N~1~-butyl-5-cyano-N~3~-{(1S,2R)-1-(3,5-difluorobenzyl)-2-hydroxy-3-[(3-methoxybenzyl)amino]propyl}-N~1~-methyl-1H-indole-1,3-dicarboxamide | C34 H37 F2 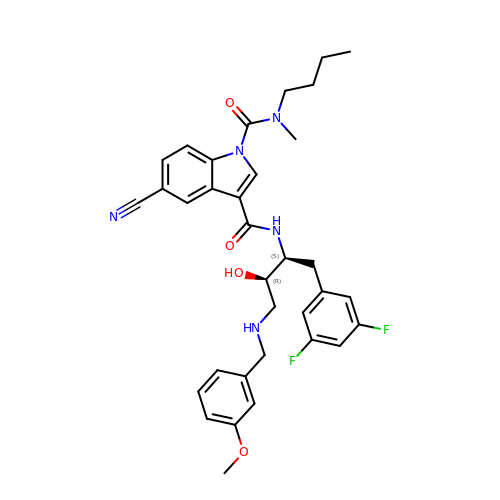N5 O4 | ZAVRTXWWDAGODB-XDFJSJKPSA-N>[2x]GPRGCPTHCHCEPDGRMLLRVDCSDLGLSELPSNLSVFTSYLDLSMNNISQLLPNPLPSLRFLEELRLAGNALTYIPKGAFTGLYSLKVLMLQNNQLRHVPTEALQNLRSLQSLRLDANHISYVPPSCFSGLHSLRHLWLDDNALTEIPVQAFRSLS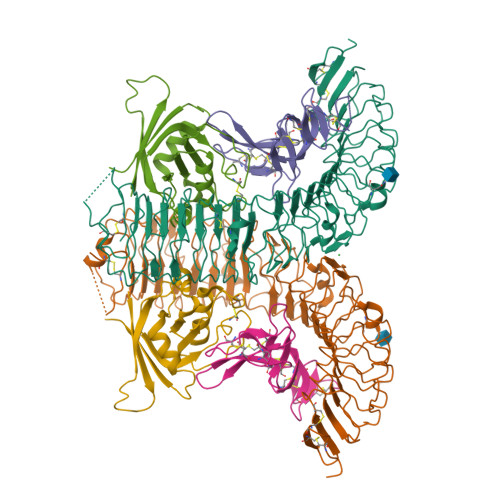ALQAMTLALNKIHHIPDYAFGNLSSLVVLHLHNNRIHSLGKKCFDGLHSLETLDLNYNNLDEFPTAIRTLSNLKELGFHSNNIRSIPEKAFVGNPSLITIHFYDNPIQFVGRSAFQHLPELRTLTLNGASQITEFPDLTGTANLESLTLTGAQISSLPQTVCNQLPNLQVLDLSYNLLEDLPSFSVCQKLQKIDLRHNEIYEIKVDTFQQLLSLRSLNLAWNKIAIIHPNAFSTLPSLIKLDLSSNLLSSFPITGLHGLTHLKLTGNHALQSLISSENFPELKVIEMPYAYQCCAFGVCENAYKISNQWNKGDNSSMDDLHKKDAGMFQAQDERDLEDFLLDFEEDLKALHSVQCSPSPGPFKPCEHLLDGAAA;>GPQKAIIRVIPLKMDPTGKLNLTLEGVFAGVAEITPAEGKLMQSHPLYLCNASDDDNLEPGFISIVKLESPRRAPRPCLSLASKARMAGERGASAVLFDITEDRAAAEQLQQPLGLTWPVVLIWGNDAEKLMEFVYKNQKAHVRIELKEPPAWPDYDAAA[2x];>GPEGSQACAKGCELCSEVNGCLKCSPKLFILLERNDIRQVGVCLPSCPPGYFDARNPDMNKCIKCKIEHCEACFSHNFCTKCKEGLYLHKGRCYPACPEGSSAANGTMECSSAAA[2x]>[4x]SMGGTLFEVVKLGKSAMQSVVDDWIESYKQDRDIALLDLINFFIQCSGCRGTVRIEMFRNMQNAEIIRKMTEEFDEDSGDYPLTMPGPQWKKFRSNFCEFIGVLIRQCQYSIIYDEYMMDTVISLLTGLSDSQVRAFRH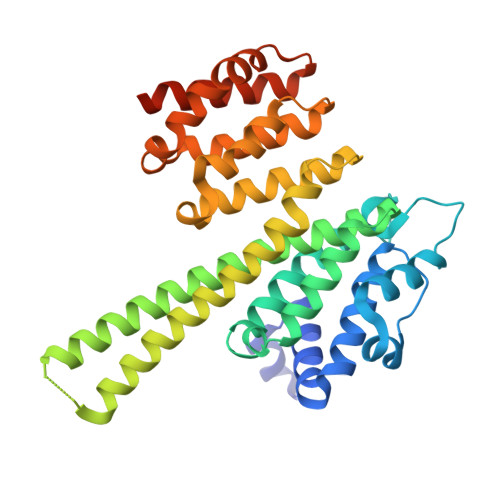TSTLAAMKLMTALVNVALNLSIHQDNTQRQYEAERNKMIGKRANERLELLLQKRKELQENQDEIENMMNSIFKGIFVHRYRDAIAEIRAICIEEIGVWMKMYSDAFLNDSYLKYVGWTLHDRQGEVRLKCLKALQSLYTNRELFPKLELFTNRFKDRIVSMTLDKEYDVAVEAIRLVTLILHGSEEALSNEDCENVYHLV>SMKLDIKKTFSNRSDRVAGIDFHPTEPWVLTTLYSGRVEIWNYETQVEVRSIQVTETPVRAGKFIARKNWIIVGSDDFRIRVFNYNTGEKVVDFEAHPDYIRSIAVHPTKPYVLSGSDDLTVKLWNWENNWALEQTFEGHEHFVMCVAFNPKDPSTFASGCLDRTVKVWSLGQSTPNFT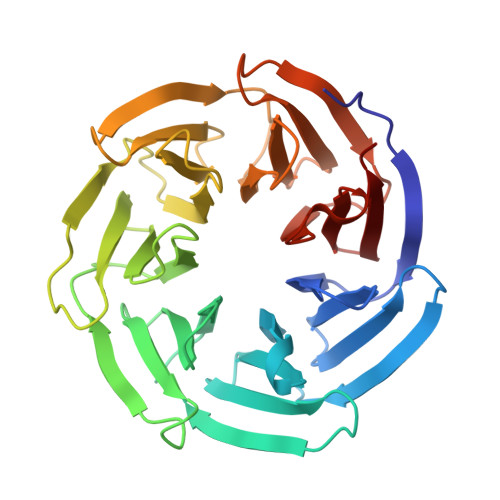LTTGQERGVNYVDYYPLPDKPYMITASDDLTIKIWDYQTKSCVATLEGHMSNVSFAVFHPTLPIIISGSEDGTLKIWNSSTYKVEKTLNVGLERSWCIATHPTGRKNYIASGFDNGFTVLSLG[2x]The first documented single-component Trp-FDH is AetF from cyanobacterium *Aetokthonos hydrillicola*, which catalyzes consecutively bromination on C5 and then C7 of Trp to generate 5,7-di-Br-Trp. More recently, a class of “single-component” FDHs has been identified. These enzymes fuse pyridine nucleotide-dependent flavin reductase and FDH on the same polypeptide chain, an advantageous feature in the application aspect relative to canonical FDHs owing to the omission of including a flavin reductase. The action of FDHs requires the reduced flavin and molecular oxygen to generate hydroperoxyl flavin intermediate, which oxidizes a halide ion to form a halogenating reagent hypohalous acid (HOX). The flipping allows the carbon-to-be-halogenated to be oriented toward the catalytic residue K258 and within the hydrogen bond distance to the putative general base E200, such that the halogenation site on two substrates is switched from C5 to C7.

We also inspected the structure of AetF in complex with 5-Br-Trp and found that V220 is in close vicinity to the Br on C5 (**[Fig fig1]**). We thus substituted V220 with bulkier residues including Ile and Leu in an attempt to reduce the enzyme’s capability in binding 5-Br-Trp. Unlike AetF-S523A, no di-brominated Trp was detectable in all doublets with AetF-V220I/S523A, hereinafter termed AetF-AI, being the most effective variant, whose 5-Br-Trp production is 3.2-fold higher than the wild type enzyme (**[Fig fig1]**). Compared with the wild type enzyme, AetF-AI exhibits much lower activity against 5-Br-Trp but approximately 25 % substrate conversion occurred in 8 hrs, suggesting that the variant still possesses C7 halogenase activity. The crystal structure of AetF-AI in complex with Trp was solved to reveal the substrate-binding mode to facilitate the subsequent rationale design (**[Table tbl1] and [Fig fig2]**). The substrate was found to bind to the same location as those in the WT and AetF-S523A, suggesting that the substitution of V220 with Ile marginally, if any, influences the substrate-binding pose (**Fig. S2**). As the case of AetF-S523A, we failed to obtain the complex structure of AetF-AI and 5-Br-Trp. Therefore, we assessed the putative binding pose of 5-Br-Trp by modeling 5-Br-Trp from the AetF/5-Br-Trp complex structure to the crystal structure of AetF-AI/Trp (**[Fig fig2]**). From this model, the side chain of I220 is distant from the Br on 5-Br-Trp by only 2.2 Å, a distance that may exclude the binding of 5-Br-Trp. Based on these analyses, we considered that additional steric hindrance in the vicinity of Br on the 5-Br-Trp may assist to reduce the binding of 5-Br-Trp so as the production of 5,7-di-Br-Trp of AetF-AI.

> MLEVCIIGFGFSAIPLVRELARTQTEFQIISAESGSVWDRLSESGRLDFSLVSSFQTSFYSFDLVRDYEKDYYPTAKQFYEMHERWRSVYEEKIIRDFVTKIENFKDYSLISTRSGKTYEAKHVVLATGFDRLMNTFLSNFDNHVSNKTFVFDTMGDSANLLIAKLIPNNNKIILRTNGFTALDQEVQVLGKPFTLDQLESPNFRYVSSELYDRLMMSPIYPRTVNPAVSYNQFPLIRRDFSWVDSKSSPPNGLIAIKYWPIDQYYYHFNDDLENYISKGYLLNDIAMWLHTGKVILVPSDTPINFDKKTITYAGIERSFHQYVKGDAEQPRLPTILINGETPFEYLYRDTFMGVIPQRLNNIYFLGYTRPFTGGLANITEMQSLFIHKLITQPQFHQKIHQNLSKRITAYNQHYYGAAKPRKHDHTVPFGFYTEDIARLIGIHYQPNECRSVRDLLFYYAFPNNAFKYRLKGEYAVDGVDELIQKVNDKHDHYAQVFVQALSIRNMNSDEAAEWDHSARRFAFNDMRHKEGYRAFLDTYLKAYRQVENISVDDTVVDEEWNFMVKEACQVRDKVAPNIEEKTHYSKDEDVNKGIRLILSILDSDISSLPDSNGSRGSGNLKEGDRLCKFEAQSIEFIRRLLQPKNYELLFIRESTVSPGSHRHGETA> MTNPVFNGKALTLKQKVGQLVMAGFNGLEASDDARKLITEDHVGGIIYFRRNLAEPAQVAKLSAELQQIAAESDNVPLLISIDQEGGMVTRLENGVTVVPGNMALGAAGDAELAYEAAHIIGSELRALGINMNFAPSLDINNNPGNPVIGVRSYGGTAELVARLGTEAVRGFQDAGVAATVKHFPGHGDTGEDSHHALPTVPHARERLDRLELAPFREAIARGVDAVMTAHVLFPAVEPEKLPATLSSNVIEGL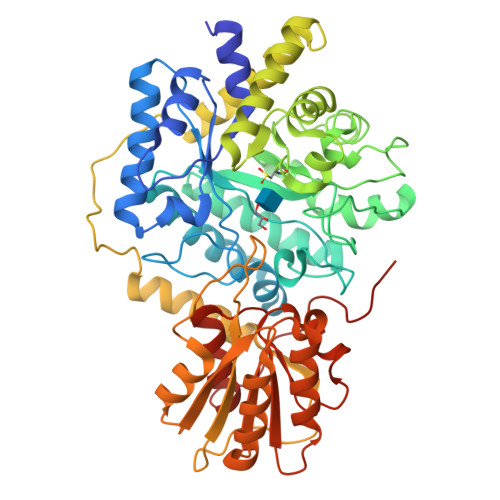LRGELGYDGVVVTDCLEMNAISKFYGVGEGAVQAVEAGADLILVSHRYERQKAALDALLAAVESGRISEERIDRSVGRLLALKQRRAVDAGAAVTLSSGDTLVTDEKTELVERISEKSITLLRSEGEFTLDKTKPVLVVWPEVRVGSEVDEVLPRKETLGYWLKSAGYDVNEQTIGVQPTEEEVAHIQELSGQISQVVVVSYNAIFSPDQAALIEALAAKPDVQLIVASARNPFDINALPTVKTFFAAYENTPSAMRALALVLTGQIAVQGTLPAPLTVTV>GIGDPVTCLKSGAICHPVFCPRRYKQIGTCGLPG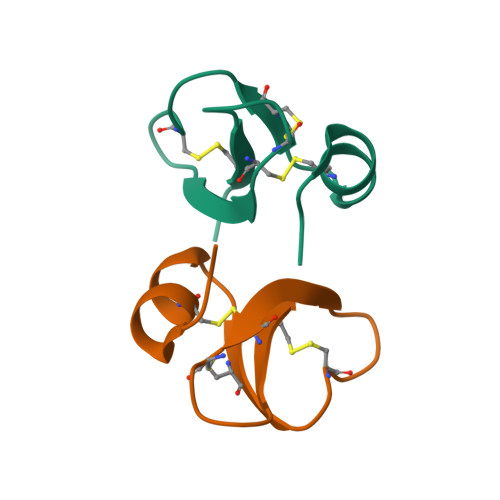TKCCKKP[4x]> GTTPSPVPTTSTCS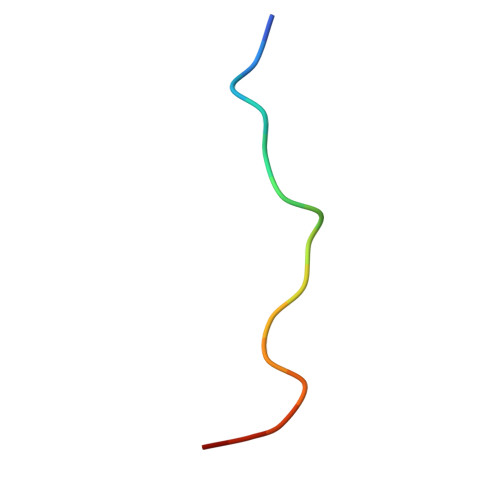AA>SNAAESSYMGKHWTEKSLHEMNERDWRILKEDYAIVTKGGTVENPLRNWEELNIIPRDLLRVIIQELRFPSPTPIQRITIPNVCNMKQYRDFLGVASTGSGKTLAFVIPILIKMSRSPPRPPSLKIIDGPKALILAPTRELVQQIQKETQKVTKIWSKESNYDCKVISIVGGHSLEEISFSLSEGCDILVATPGRLIDSLENHLLVMKQVETLVLDEADKMIDLGFEDQVTNILTKVDINADSAVNRQTLMFTATMTPVIEKIAAGYMQKPVYATIGVETGSEPLIQQVVEYADNDEDKFKKLKPIVAKYDPPIIIFINYKQTADWLAEKFQKETNMKVTILHGSKSQEQREHSLQLFRTNKVQIMIATNVAARGLDI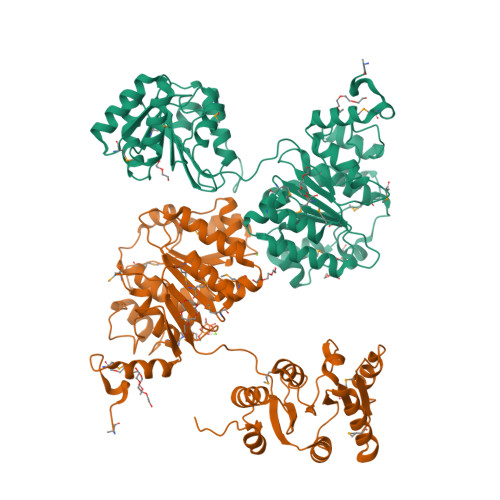PNVSLVVNFQISKKMDDYIHRIGRTGRAANEGTAVSFVSAAEDESLIRELYKYVRKHDPLNSNIFSEAVKNKYNVGKQLSNEIIY[2x]Volume-regulated anion channels (VRACs) are hexamers of LRRC8 proteins that are crucial for cell volume regulation. An LRRC8 subunit consists of an amino terminus (NT), four transmembrane helices, and a carboxyterminal LRR (leucine-rich repeat) domain. Recent cryo-EM studies of LRRC8A, LRRC8D, and LRRC8A/C channels reveal a hexameric assembly of LRRC8 subunits around the central axis of symmetry that defines the ion conduction pore. LRRC8 channels can be activated by low ionic strength and cell swelling.

Here, we present the 2.8-Å cryo-EM structure of homomeric human LRRC8A (HsLRRC8A) channels that for the first time shows NTs resolved at a local resolution of 3.0–3.2 Å. The HsLRRC8A protein was heterologously overexpressed in HEK293S GnTI− cells and purified at high NaCl concentration (≥300 mM, see STAR Methods). The cryo-EM density map of HsLRRC8A achieved an overall resolution of 2.8 Å with imposed C3 symmetry. The final model was built for residues M1–W411 of the pore domain, with the exception of disordered residues F69–D91 in EL1 and residues V177–G230 of the intracellular loop IL1. Concordant with an accessibility analysis, the NTs, resolved at 3.0- to 3.2-Å resolution, locate at the inner surface of the pore domain and span nearly the entire width of the membrane. However, the NT (M1–L20) of HsLRRC8A channels can be partitioned into four subsegments, which we named NTa (loop, M1–P3), NTb (310 helix, V4–F10), NTc (loop, A11–Q14), and NTd (310 helix, P15–L20). In the present structure with resolved NTs, the permeation path is partitioned into a neck and a base. The neck, with an average diameter of approximately 11.2 Å, is lined by residues of the N-halves of the NTs and by residues of the extracellular halves of TM1. The narrowest portion of the neck is situated at residues M1, P3, and T5, where it displays diameters of about 10.3, 10.3, and 10.2 Å, respectively. Although the narrowest portion of the neck is wide enough for the passage of hydrated halide anions (∼7.0 Å), it is narrower than the size (11.0–13.0 Å) required for the experimentally determined passage of larger anions and molecules in native VRACs. This suggests that the pore may be in a partially closed state and undergoes further dilation when channels are fully opened.

>[6x]MIPVTELRYFADTQPAYRILKPWWDVFTDYISIVMLMIAVFGGTLQVTQDKMICLPCKWVTKDSCNDSFRGWAAPGPEPTYPNSTILPTPDTGPTGIKYDLDRHQYNYVDAVCYENRLHWFAKYFPYLVLLHTLIFLACSNFWFKFPRTSSKLEHFVSILLKCFDSPWTTRALSETVVEESDPKPAFSKMNGSMDKKSSTVSEDVEATVPMLQRTKSRIEQGIVDRSETGVLDKKEGEQAKALFEKVKKFRTHVEEGDIVYRLYMRQTIIKVIKFILIICYTVYYVHNIKFDVDCTVDIESLTGYRTYRCAHPLATLFKILASFYISLVIFYGLICMYTLWWMLRRSLKKYSFESIREESSYSDIPDVKNDFAFMLHLIDQYDPLYSKRFAVFLSEVSENKLRQLNLNNEWTLDKLRQRLTKNAQDKLELHLFMLSGIPDTVFDLVELEVLKLELIPDVTIPPSIAQLTGLKELWLYHTAAKIEAPALAFLRENLRALHIKFTDIKEIPLWIYSLKTLEELHLTGNLSAENNRYIVIDGLRELKRLKVLRLKSNLSKLPQVVTDVGVHLQKLSINNEGTKLIVLNSLKKMANLTELELIRCDLERIPHSIFSLHNLQEIDLKDNNLKTIEEIISFQHLHRLTCLKLWYNHIAYIPIQIGNLTNLERLYLNRNKIEKIPTQLFYCRKLRYLDLSHNNLTFLPADIGLLQNLQNLAITANRIETLPPELFQCRKLRALHLGNNVLQSLPSRVGELTNLTQIELRGNRLECLPVELGECPLLKRSGLVVEEDLFNTLPPEVKERLWRADKE> MASKAIVQMAKILRKELSEE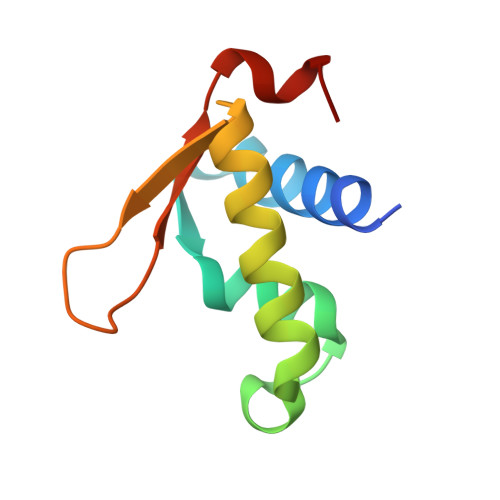KEVIFTDVLKSQANTEPENITKREASRGFFDILSLATEGCIGLSQTEAFGNIKIDAKPALFERFI The large family of Gram-positive quorum-sensing receptors known as the RNPP proteins consists of receptors homologous to the Rap, NprR, PlcR, and PrgX proteins that are regulated by imported oligopeptide autoinducers. Rap proteins are phosphatases and transcriptional anti-activators, and NprR, PlcR, and PrgX proteins are DNA binding transcription factors. Rap proteins and their inhibitory oligopeptides, called Phr peptides, have been most extensively studied in B. subtilis, which encodes 11 Rap proteins on its chromosome and another five on plasmids. Sequence and structural analysis shows that the Rap proteins are repeat proteins consisting of nine HTH TPR or TPR-like folds, which pack together to form a right-handed superhelical TPR domain.

Following the discovery that RapJ and PhrC form a regulatory pair, we crystallized and determined the 2.16 Å resolution X-ray crystal structure of the RapJ-PhrC complex. Readily interpretable electron density corresponding to each residue in the PhrC pentapeptide was observed, and PhrC was modeled only after the RapJ model was nearly complete. Relative to its position in the RapH-Spo0F and RapF-ComAC structures, the entire N-terminal 3-helix bundle and linker region have dramatically flipped and repacked against the N-terminal surface of the C-terminal TPR domain in the RapJ-PhrC structure. In fact, the RapJ 3-helix bundle (residues 1–70) and helix-containing linker region (residues 71–94) merge with the C-terminal TPR domain (residues 95–373) to form one extended TPR domain (residues 1–373). In contrast, in the RapJ-PhrC structure, the ligand-binding groove is closed. PhrC binding stabilizes a closed RapJ conformation that differs from the open RapI conformation due to a compression of RapJ along the TPR superhelical axis. The RapJ-PhrC structure revealed that RapJ residue Asp192 forms a salt-bridge with PhrC residue Arg2. RapJ-PhrC interface mutations E147A, Y150F, D192A, N225A, F250A, and K300E resulted in a complete loss of sensitivity to PhrC and, together with previous mutagenesis studies, confirm the biological importance of the crystallographically identified RapJ-PhrC interface. New intramolecular RapJ contacts that form as a result of the PhrC-induced compression stabilize the RapJ closed conformation and are necessary for PhrC inhibition of RapJ Spo0F phosphatase activity.

>MRAKIPSEEVAVKLNEWYKLIRAFEADQAEALKQEIEYDLEDMEENQDLLLYFSLMEFRHRIMLDKLMPVKDSDTKPPFSDMLNEIESNQQKLTGLLEYYFYYFRGMYEFKQKNFILAIDHYKHAEEKLEYVEDEIEKAEFLFKVAEVYYHIKQTYFSMNYASQALDIYTKYELYGRRRVQCEFIIAGNLTDVYHHEKALTHLCSALEHARQLEEAYMIAAAYYNVGHCKYSLGDYKEAEGYFKTAAAIFEEHNFQQAVQAVFSLTHIYCKEGKYDKAVEAYDRGIKSAAEWEDDMYLTKFRLIHELYLGSGDLNVLTECFDLLESRQLLADAEDLLHDTAERFNQLEHYESAAFFYRRLMNIKKKLAEQRFQ[2x];>[2x]ERGMT>[2x]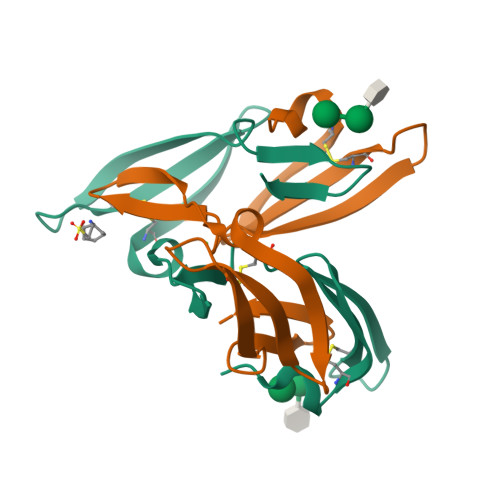LGKFSQTCYNSAIQGSVLTSTCERTNGGYNTSSIDLNSVIENVDGSLKWQPSNFIETCRNTQLAGSSELAAECKTRAQQFVSTKINLDDHIANIDGTLKYE> SSSLKIASTQEARQYFDTDRVVVDAVGSDFTDVGAVIAMDYETDVIDAADATKFGIPVFAVTKDAQAISADELKKIFHIIDLENKFDATVNAREIETAVNNYEDSILPPFFKSLKEYVSRYLIQFDCPGHQGGQYYRKHPAGREFYDFFGETVFRADLCNADVALGDLLIHEGPAVAAEKHAARVYNADKTYFVLGGSSNANNTVTSALVSNGDLVLFDRNNHKSVYNSALAMAGGRPVYLQTNRNPYGFIGGIYDSDFDEKKIRELAAKVDPERAKWKRPFRLAVIQLGTYDGTIYNAHEVVKRIGHLCDYIEFDSAWVGYEQFIPMMRNSSPL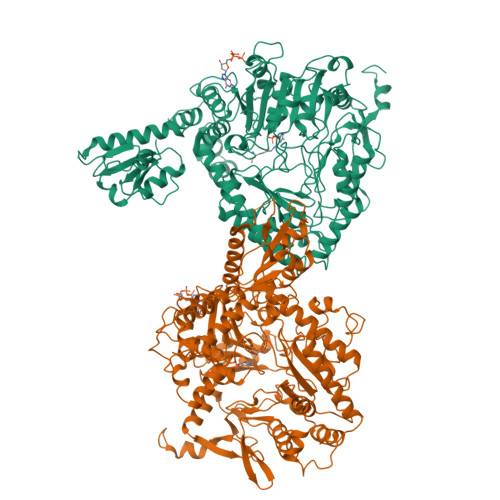LIDDLGPEDPGIIVVQSVHKQQAGFSQTSQIHKKDSHIKGQLRYCDHKHFNNSFNLFMSTSPFYPMYAALDVNAAMQEGEAGRKLWHDLLITTIEARKKLIKAGSMFRPFVPPVVNGKKWEDGDTEDMANNIDYWRFEKGAKWHAYEGYGDNQYYVDPNKFMLTTPGINPETGDYEDFGVPATIVANYLRDHGIIPEKSDLNSILFLMTPAETPAKMNNLITQLLQLQRLIEEDAPLKQVLPSIYAANEERYNGYTIRELCQELHDFYKNNNTFTYQKRLFLREFFPEQGMLPYEARQEFIRNHNKLVPLNKIEGEIALEGALPYPPGVFCVAPGEKWSETAVKYFTILQDGINNFPGFAPEIQGVYFKQEGDKVVAYGEVYDAEVAKNDDRYNN Rotaviruses are the leading etiologic agent of viral gastroenteritis in infants and young children worldwide and are responsible for an estimated 140,000 deaths each year in developing countries. Diverse interactions between histo-blood group antigens (HBGAs) and rotavirus have been described and it is believed that HBGAs expressed on the surface of target cells serve as viral receptors. The distal VP8* portion (~27 kDa, N-terminal) of the rotavirus spike protein VP4 from P, P, P and P genotypes recognize the secretor HBGAs. To understand the molecular basis of LNB and H1 recognition and binding to P VP8* we determined the crystal structure of the clinical isolate P[8]c VP8* in its apo form and bound to LNB and H1 glycans.

Two different crystalline forms of P[8]c VP8* in its apo form were obtained. The first form, VP8*-Apo1, diffracts at 1.35 Å resolution and presents a single copy of P[8]c VP8* in the crystal asymmetric unit (ASU) while the second form, VP8*-Apo2, diffracts to 1.5 Å and presents two copies in the ASU. The three copies of P[8]c VP8* in these two crystalline forms present the galectin fold with two twisted β-sheets separated by a superficial cleft that conforms the glycan binding site in P and P genotypes. Superimposition of the individual VP8* protomers from these crystals showed that the three molecules of P[8]c VP8* are almost identical (RMSD 0.28 Å for the superposition of all the Cα). Furthermore, P[8]c VP8* are also structurally identical (RMSDs 0.37–0.57 Å) to the VP8* apo forms of the linage I P[8]Wa and P[8]Rotarix, supporting that the glycan binding site is preformed in the P[8]c VP8* protein.

>[2x]GSMLDGPYQPTTFTPPSDYWILINSNTNGVVYESTNNSDFWTAVIAVEPHVDPVDRQYNVFGENKQFNVRNDSDKWKFLEMFRGSSQNDFYNRRTLTSNTRLVGILKYGGRIWTFHGETPRATTDSSNTANLNGISITIHSEFYIIPRSQESKCNEYINNGL>MDHHHHHHDTGQSQTQRMYNYLKAKYTATSGTQLAWGAYLDPVDGNPSSVYAEFDERAHNVDPSTEPIKSTHTFKDGSVAEIEMNGQLVDGLTGPENYN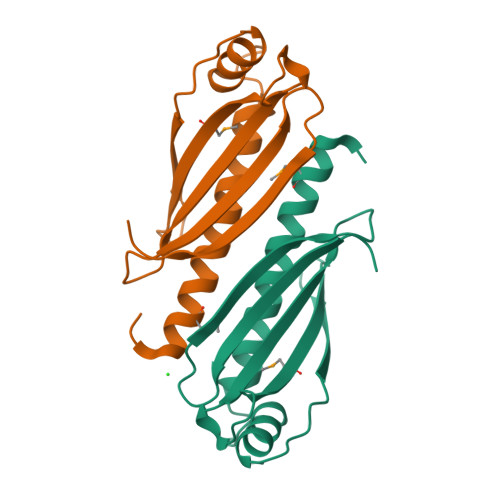ITIKSKSKLAGSNDYYEHIVTFNFDTKGIRSEEGHLRSAQK[4x]> MEYEWKPDEQGLQQILQLLKE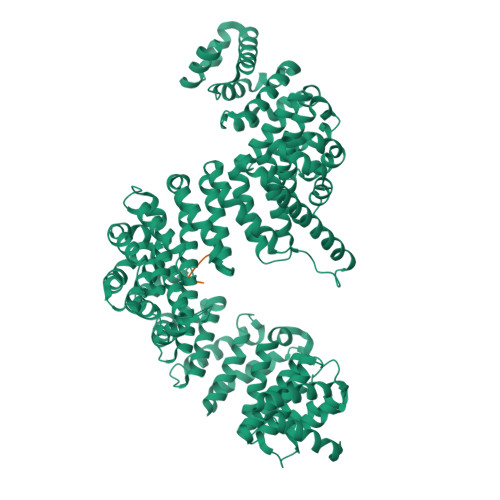SQSPDTTIQRTVQQKLEQLNQYPDFNNYLIFVLTKLKSEDEPTRSLSGLILKNNVKAHFQNFPNGVTDFIKSECLNNIGDSSPLIRATVGILITTIASKGELQNWPDLLPKLCSLLDSEDYNTCEGAFGALQKICEDSAEILDSDVLDRPLNIMIPKFLQFFKHSSPKIRSHAVACVNQFIISRTQALMLHIDSFIENLFALAGDEEPEVRKNVCRALVMLLEVRMDRLLPHMHNIVEYMLQRTQDQDENVALEACEFWLTLAEQPICKDVLVRHLPKLIPVLVNGMKYSDIDIILLKGDVEGGSGGSGDDTISDWNLRKCSAAALDVLANVYRDELLPHILPLLKELLFHHEWVVKESGILVLGAIAEGCMQGMIPYLPELIPHLIQCLSDKKALVRSITCWTLSRYAHWVVSQPPDTYLKPLMTELLKRILDSNKRVQEAACSAFATLEEEACTELVPYLAYILDTLVFAFSKYQHKNLLILYDAIGTLADSVGHHLNKPEYIQMLMPPLIQKWNMLKDEDKDLFPLLECLSSVATALQSGFLPYCEPVYQRCVNLVQKTLAQAMLNNAQPDQYEAPDKDFMIVALDLLSGLAEGLGGNIEQLVARSNILTLMYQCMQDKMPEVRQSSFALLGDLTKACFQHVKPCIADFMPILGTNLNPEFISVCNNATWAIGEISIQMGIEMQPYIPMVLHQLVEIINRPNTPKTLLENTAITIGRLGYVCPQEVAPMLQQFIRPWCTSLRNIRDNEEKDSAFRGICTMISVNPSGVIQDFIFFCDAVASWINPKDDLRDMFCKILHGFKNQVGDENWRRFSDQFPLPLKERLAAFYGV;> RFTQRGGGAVGKNRRGGRGGNRGGRNNNSTRFNPLAKA>[16x]SVDHGFLVTRHSQTTDDPQCPPGTKILYHGYSLLYVQGNERAHGQDLGTAGSCLRKFSTMPFLFCNINNVCNFASRNDYSYWLSTPEPMPMSMAPITGENIRPFISRCAVCEAPAMVMAVHSQTIQIPQCPTGWSSLWIGYSFVMHTSAGAEGSGQALASPGSCLEEFRSAPFIECHGRGTCNYYANAYSFWLATIERSEMF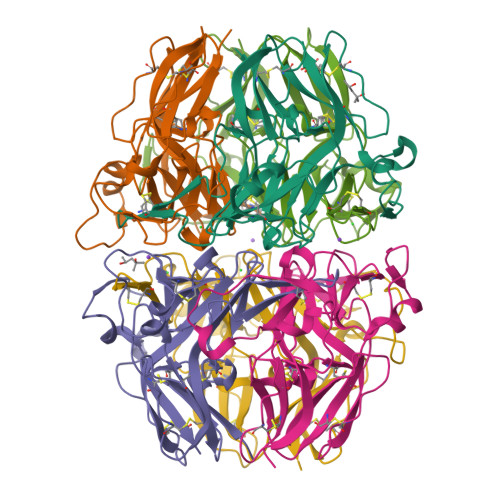KKPTPSTLKAGELRTHVSRCQVCMRRT;>[8x]ISIGYLLVKHSQTDQEPMCPVGMNKLWSGYSLLYFEGQEKAHNQDLGLAGSCLARFSTMPFLYCNPGDVCYYASRNDKSYWLSTTAPLPMMPVAEEDIRPYISRCSVCEAPAVAIAVHSQDVSIPHCPAGWRSLWIGYSFLMHTAAGDEGGGQSLVSPGSCLEDFRATPFIECNGARGTCHYYANKYSFWLTTIPEQSFQGTPSADTLKAGLIRTHISRCQVCMKNL N-[2-(2,4-dichlorophenyl)ethyl]-2-{8-[(2,4-dimethoxyphenyl)carbonyl]-4-oxo-1-phenyl-1,3,8-triazaspiro[4.5]dec-3-yl}acetamide 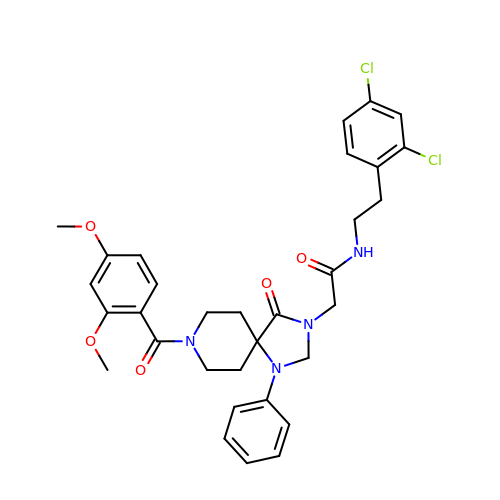| C32 H34 Cl2 N4 O5 | TWOVSEVREOPZGM-UHFFFAOYSA-N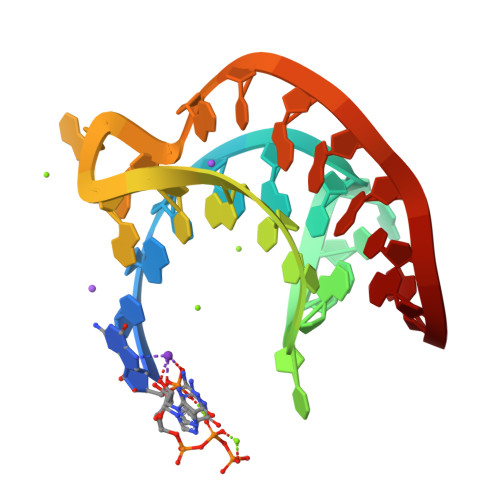> GGCGCGGCACCGUCCGCGGAACAAACGG>GNNVVVLGTQWGDEGKGKIVDLLTERAKYVVRYQGGHNAGHTLVINGEKTVLHLIPSGILRENVTSIIGNGVVLSPAALMKEMKELEDRGIPVRERLLLSEACPLILDYHVALDNAREKARGAKAIGTTGRGIGPAYEDKVARRGLRVGDLFDKETFAEKLKEVMEYHNFQLVNYYKAEAVDYQKVLDDTMAVADILTSMVVDVSDLLDQARQRGDFVMFEGAQGTLLDIDHGTYPYVTSSNTTAGGVATGSGLGPRYVDYVLGILKAYSTRVGAGPFPTELFDETGEFLCKQGNEFGATTGRRRRTGWLDTVAVRRAVQLNSLSGFCLTKLDVLDGLKEVKLCVAYRMPDGREVTTTPLAADDWKGVEPIYETMPGWSESTFGVKDRSGLPQAALNYIKRIEELTGVPID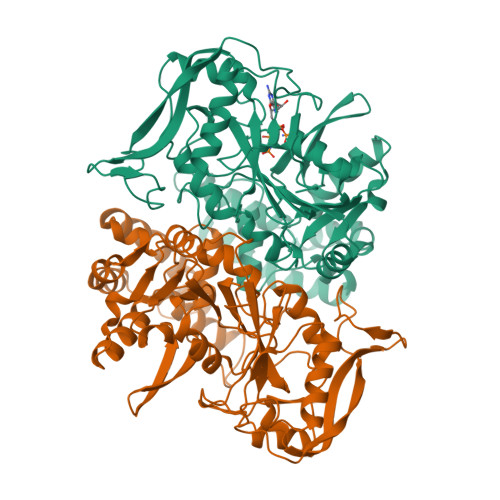IISTGPDRTETMILRDPFDA[2x]> PSTKEHFAREYDCYGDSYFIDTDLNQL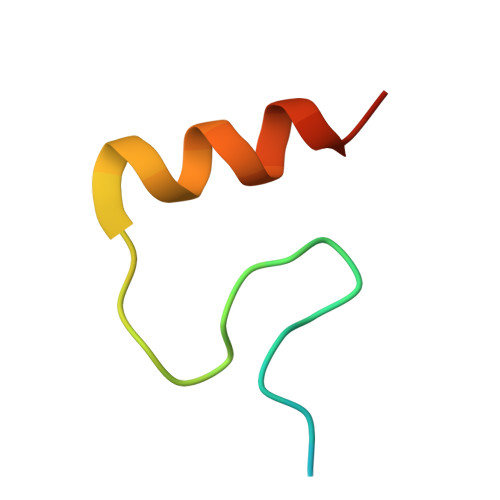KEVFSGIKNS> GHMPAHTTHDAARDEAVAPLLRGIAVLGRLTGADGGTLSLSALERTTGLARSTVDRLTATLARMGYVRLDGRDVVLAPRLMELGNAYLAALRLPALLSARADGLADELDESVSLAVGDRDGIRFIHQATRRRAMSLSFRIGDLLPAER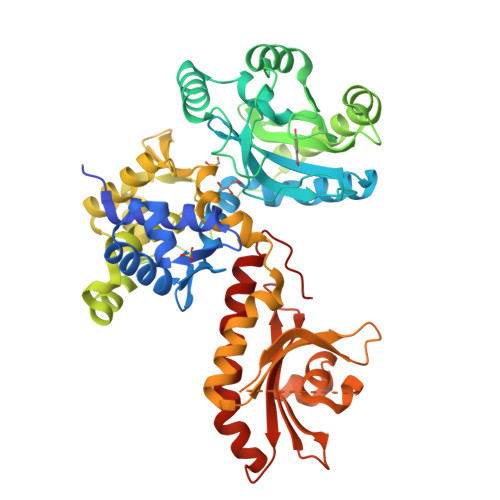TAPGPLFAAEWTASDWHRWRERRAADPGDHSFPAVPPREPGAPGEDFARRAAKAAADGWALDDQLIEPGLVAVSVPVRDPGTGRVACVASVVSHTSRHTAPDLRAALLPRLRAAVAAMEDDLRAAPAPEPGPPPAGLALWTGASKQELGREFVESLARGLTVLTAFGEGRSALTLTQVAQATGLARATARRALLTHARAGLVAPAAGHTFTLTPRVLSLGFPPLSRTSLPEIAQPHLTALAERVHESASLAVLADSGEEIQYTARASAARVLSARVTVGTRLPARATALGRVLLALPEVRARGYALVDEELEAGLRAIAVPVRDRTGRVVAALNVALHAARRTADDCVAQILPELRHTADLVETELRVAGRFCRVAVV Mycobacteria have up to five specialized secretion systems (ESX-1 to ESX-5) that transport virulence factors across their complex cell envelope to facilitate manipulation of their environment. One of these substrates, the ESX-1 secretion-associated protein B (EspB; Rv3881c), has been postulated as a structural component of the extended ESX-1 machinery. Once secreted across the inner mycobacterial membrane, EspB oligomerizes into a cylinder-like heptamer, favored by the removal of its C-terminal region and the acidic pH environment of the phagosomal lumen. EspB interacts with EspK (Rv3879c), which is encoded by a gene in the RD1 locus downstream of EspB.

An initial low resolution structure was obtained with EspB2-348 and EspK484-729 from M. tuberculosis, on the basis of which a new shorter EspB construct was designed (residues 2–300) while retaining important contact points in the crystal packing. This improved the crystal diffraction and led to a final anisotropic resolution of 2.3 Å. The crystal structure covers residues V9 to P297 for EspB, missing E87–S112 from the PE-PPE loop, whereas all residues could be built for EspK484-729. The structure resembles a sea snail, consisting of two domains. The shell consists of an antiparallel β-sheet with five peripheral α helices. The foot of the snail is formed by a compact helix bundle of three α helices with a loop containing three short helices connecting the foot with the shell. The interaction occurs between α6–7 and the PE-PPE loop of EspB and α9–10 of EspK. Analysis of the EspB-EspK interface by PISA gave an interface area of 652 Å2, ΔG of -11.7 kcal/mol, and a relative low complexation significance score of 0.1. The EspB–EspK interaction could be abolished by either shortening an amino acid side chain of EspK through a K663A substitution or by changing the hydrophobicity of a side chain through a F659D substitution in EspK, indicating that both residues are essential for complex formation. EspK binding to EspB prevents EspB oligomerization not only by steric hindrance but also by locking the PE-PPE loop, preventing it to adapt the more open conformation that is required for EspB oligomerization.

> MTQSQTVTVDQQEILNRANEVEAPMADPPTDVPITPCELTAAKNAAQQLVLSADNMREYLAAGAKERQRLATSLRNAAKAYGEVDEEAATALDNDGEGTVQAESAGAVGGDSSAELTDTPRVATAGEPNFMDLKEAARKLETGDQGASLAHFADGWNTFNLTLQGDVKRFRGFDNWEGDAATACEASLDQQRQWILHMAKLSAAMAKQAQYVAQLHVWARREHPTYEDIVGLERLYAENPSARDQILPVYAEYQQRSEKVLTEYNNKAALEPVNPPKPPPAIKIDPPPPPQEQGLIPGFL;> GDALRLARRIAAALNASDNNAGDYGFFWITAVTTDGSIVVANSYGLAYIPDGMELPNKVYLASADHAIPVDEIARCATYPVLAVQAWAAFHDMTLRAVIGTAEQLASSDPGVAKIVLEPDDIPESGKMTGRSRLEVVDPSAAAQLADTTDQRLLDLLPPAPVDVNPPGDERHMLWFELMKPMTSTATGREAAHLRAFRAYAAHSQEIALHQAHTATDAAVQRVAVADWLYWQYVTGLLDRALAAAC> PLRLGG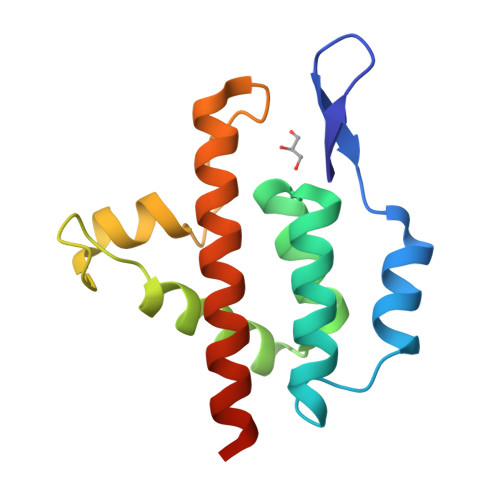NGQWQYWPFSSSDLYNWKNNNPSFSEDPGKLTALIESVLTTHQPTWDDCQQLLGTLLTGEEKQRVLLEARKAVRGNDGRPTQLPNEVDAAFPLERPDWDYTTQRGRNHLVLYRQLLLAGLQNAGRSLEHHHHHH>GAMAEHAPRRCCLGWDFSTQQVKVVAVDAELNVFYEESVHFDRDLPEFGTQGGVHVHKDGLTVTSPVLMWVQALDIILEKMKASGFDFSQVLALSGAGQQHGSIYWKAGAQQALTSL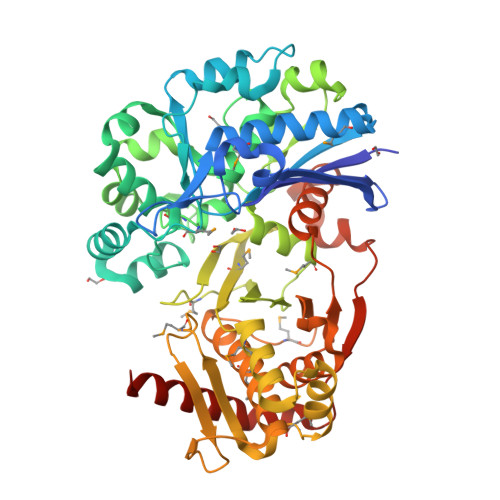SPDLRLHQQLQDCFSISDCPVWMDSSTTAQCRQLEAAVGGAQALSCLTGSRAYERFTGNQIAKIYQQNPEAYSHTERISLVSSFAASLFLGSYSPIDYSDGSGMNLLQIQDKVWSQACLGACAPHLEEKLSPPVPSCSVVGAISSYYVQRYGFPPGCKVVAFTGDNPASLAGMRLEEGDIAVSLGTSDTLFLWLQEPMPALEGHIFCNPVDSQHYMALLCFKNGSLMREKIRNESVSRSWSDFSKALQSTEMGNGGNLGFYFDVMEITPEIIGRHRFNTENHKVAAFPGDVEVRALIEGQFMAKRIHAEGLGYRVMSKTKILATGGASHNREILQVLADVFDAPVYVIDTANSACVGSAYRAFHGLAGGTDVPFSEVVKLAPNPRLAATPSPGASQVYEALLPQYAKLEQRILSQTRGPPE[3x]>[2x]MKMTKSALVTGASRGIGRSIALQ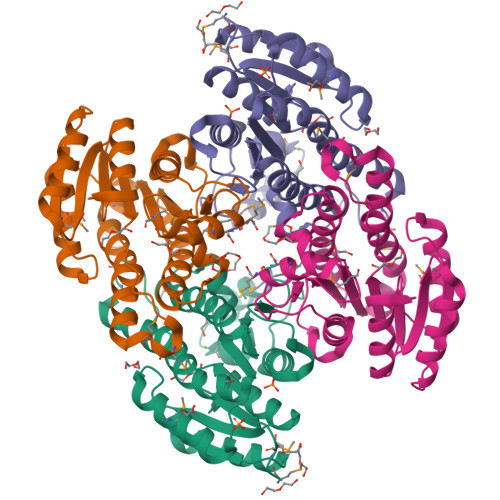LAEEGYNVAVNYAGSKEKAEAVVEEIKAKGVDSFAIQANVADADEVKAMIKEVVSQFGSLDVLVNNAGITRDNLLMRMKEQEWDDVIDTNLKGVFNCIQKATPQMLRQRSGAIINLSSVVGAVGNPGQANYVATKAGVIGLTKSAARELASRGITVNAVAPGFIVSDMTDALSDELKEQMLTQIPLARFGQDTDIANTVAFLASDKAKYITGQTIHVNGGMYM> MAAQNEQRPERIKTTPYLEGDVLSSDSGPLLSVFALQEIMQKVRQVQADYMTATREVDFTVPDVQKILDDIKALAAEQVYKIVKVPSISFRHIVMQSRDRVLRVDTYYEEMSQVGDVITEDEPEKFYSTIIKKVRFIRGKGSFILHDIPTRDHRGMEVAEPEVLGVEFKNVLPVLTAEHRAMIQNALDGSIIENGNVATRDVDVFIGACSEPVYRIYNRLQGYIEAVQLQELRNSIGWLERLGHRKRITYSQEVLTDFRRQDTIWVLALQLPVNPQVVWDVPRSSIANLIMNIATCLPTGEYIAPNPRISSITLTQRITTTGPFAILTGSTPTAQQLNDVRKIYLALMFPGQIILDLKIDPGERMDPAVRMVAGVVGHLLFTAGGRFTNLTQNMARQLDIALNDYLLYMYNTRVQVNYGPTGEPLDFQIGRNQYDCNVFRADFATGTGYNGWATIDVEYREPAPYVHAQRYIRYCGIDSRELINPTTYGIGMTYHCYNEMLRMLVAAGKDSEAAYFRSMLPFHMVRFARINQIINEDLHSVFSLPDDMFNALL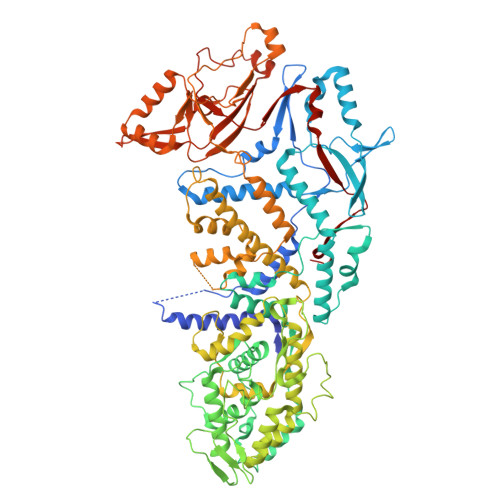PDLIAGAHQNADPVVLDVSWISLWFAFNRSFEPTHRNEMLEVAPLIESVYASELSVMKVDMRHLSLMQRRFPDVLIQARPSHFWKAVLNDSPEAVKAVMNLSHSHNFINIRDMMRWVMLPSLQPSLKLALEEEAWAAANDFEDLMLTDQVYMHRDMLPEPRLDDIERFRQEGFYYTNMLEAPPEIDRVVQYTYEIARLQANMGQFRAALRRIMDDDDWVRFGGVLRTVRVKFYDARPPDDVLQGLPFSYDTNERGGLAYATIKYATETTIFYLIYNVEFSNTPDSLVLINPTYTMTKVFINKRIVERVRVGQILAVLNRRFVAYKGKMRIMDITQSLKMGTKLAAPTV>[2x]MYRLQIEKIRGFRDFYPEDMDVEKFIFKTAEEAAEAFGFRRIDFPSLEYLDLYRIKSGEELLQQTYSFVDKGGREVTLIPEATPSTVRMVTSRKDLQRPLRWYSFPKVWRYEEPQAGRYREHYQFNADIFGSDSPEADAEVIALASSILDR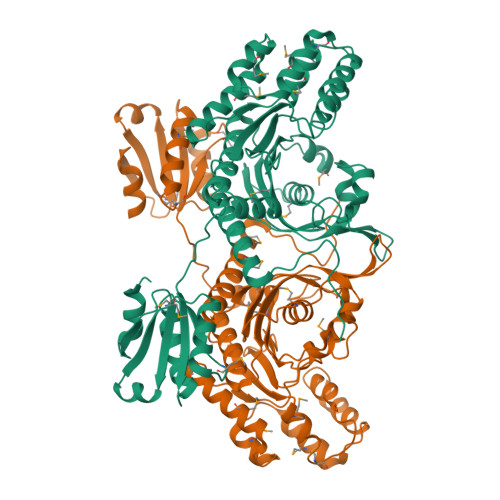LGLQDIYEIRINSRKIMEEIIGGMTSSDPFSVFSIIDRYHKISREEFVDQLRSAGIGEDGVSMIADLCSGTRGIDEMARITGKSSEEIARMAAVEDLLASYGVKNVRYDFSIVRGLSYYTGIVFEAYDRSGQFRAILGGGRYDNLASLMSGESVPAVGFGMGDAVISLLLKRENVQIPREKKSVYICRVGKINSSIMNEYSRKLRERGMNVTVEIMERGLSAQLKYASAIGADFAVIFGERDLERGVVTIRNMYTGSQENVGLDSVVEHLISQATLEHHHHHH> GSPQAHPVPKDARITHSSGQSFEQMRQECLQRGTLFEDADFPASNSSLFYSERPQIPFVWKRPGEIVKNPEFILGGATRTDICQGELGDCWLLAAIASLTLNQKALARVIPQDQSFGPGYAGIFHFQFWQHSEWLDVVIDDRLPTFRDRLVFLHSAD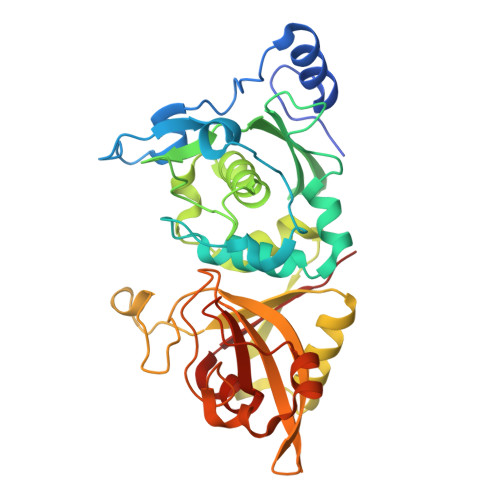HNEFWSALLEKAYAKLNGSYEALKGGSAIEAMEDFTGGVAETFQTKEAPENFYEILEKALKRGSLLGCFIDTRSAAESEARTPFGLIKGHAYSVTGIDQVSFRGQRIELIRIRNPWGQVEWNGSWSDSSPEWRSVGPAEQKRLCHTALDDGEFWMAFKDFKAHFDKVEICNLTPDA> MWNVVGQIIS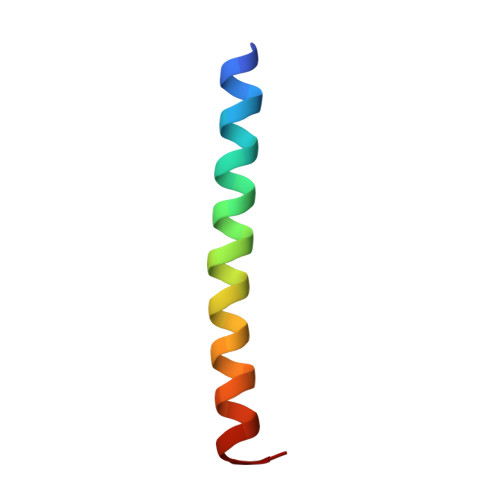VLCFFILTVGTLFGIVYVSHLLSRG> MHHHHHHMPIIEQVRAREILDSRGNPTVEVEVALIDGTFARAAVPSGASTGEHEAVELRDGGDRYGGKGVQKAVQAVLDEIGPA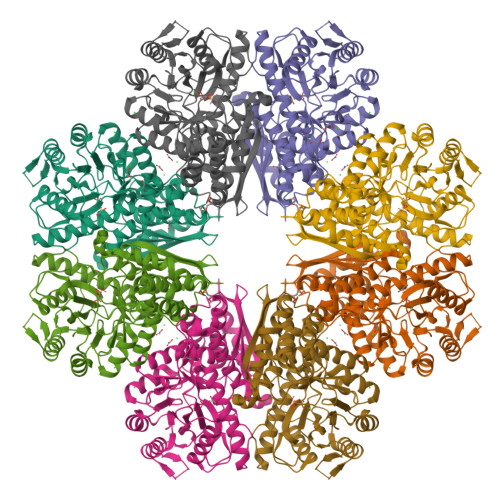VIGLNADDQRLVDQALVDLDGTPDKSRLGGNAILGVSLAVAKAAADSAELPLFRYVGGPNAHILPVPMMNILNGGAHADTAVDIQAFMVAPIGAPSFVEALRWGAEVYHALKSVLKKEGLSTGLGDEGGFAPDVAGTTAALDLISRAIESAGLRPGADVALALDAAATEFFTDGTGYVFEGTTRTADQMTEFYAGLLGAYPLVSIEDPLSEDDWDGWAALTASIGDRVQIVGDDIFVTNPERLEEGIERGVANALLVKVNQIGTLTETLDAVTLAHHGGYRTMISHRSGETEDTMIADLAVAIGSGQIKTGAPARSERVAKYNQLLRIEEALGDAARYAGDLAFPRFACETK>MAYFLEQTDSEIFELIFEEYKRQNEHLEMIASENYTFASVMEAMGSVLTNKYAEGYPNKRYYGGCEVVDKIESLAIERAKKLFNCQFANVQAHSGSQANNAVYHALLKPYDKILGMDLSCGGHLTHGAKVSLTGKHYQSFSYGVNLDGYIDYEEALKIAQSVKPEIIVCGFSAYPREIDFKKFREIADEVGALLLGDIAHVAGLVVTGEHAHPFPHCHVVSSTTHKTLRGPRGGIILTNDEEIAAKIDKAIFPGTQGGPLMHVIAAKAVGFKENLKPEFKAYAQLVKSNMQVLAKALKEKNHKLVSGGTSNHLLLMDFLDKPYSGKDADIALGNAGITVNKNTIPGETRSPFVTSGIRIGSAALSARGMGAKEFEIIGNKIS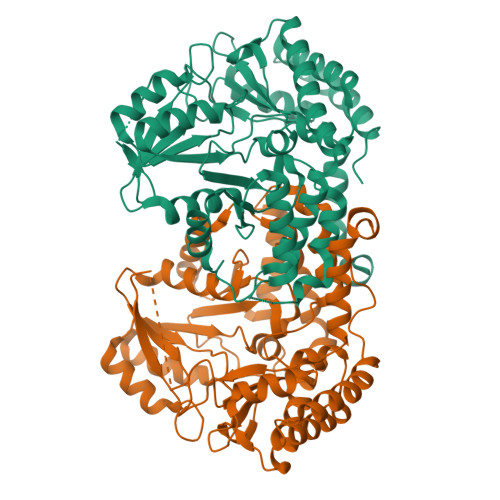DILNDINNVSLQLHVKEELKAMVNQFPVYHQPIFRSHHHHHH[2x]> MTGYLTIGGQRYQAEINDLENLGEMGSGTCGQVWKMRFRKTGHVIAVKQMRRSGNKEENKRILMDLDVVLKSHDCPYIVQCFGTFITNTDVFIAMELMGTCAEKLKKRMQGPIPERILGKMTVAIVKALYYLKEKHGVIHRDVKPSNILLDERGQIKLSDFGISGRLVDSKAKTRSAGCAAYMAPERIDPPDPTKPDYDIRADVWSLGISLVELATGQFPYKNCKTDFEVLTKVLQEEPPLLPGHMGFSGDFQSFVKDCLTKDHRKRPKYNKLLEHSFIKRYETLEVDVASWFKDVMAKTESPR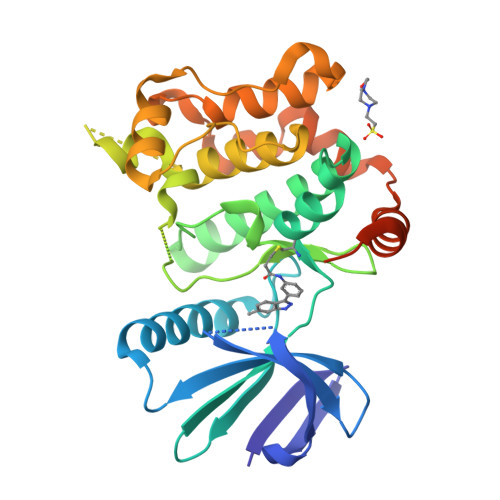TSGVLSQPHLPFFRHHHHHH>MREKGRRQAVRGPAFMFNDRGTSLTAEEERFLDAAEYGNIPVVRKMLEESKTLNVNCVDYMGQNALQLAVGNEHLEVTELLLKKENLARIGDALLLAISKGYVRIVEAILNHPGFAASKRLTLSPCEQELQDDDFYAYDEDGTRFSPDITPIILAAHCQKYEVVHMLLMKGARIERPHDYFCKCGDCMEKQRHDSFSHSRSRINAYKGLASPAYLSLSSEDPVLTALELSNELAKLANIEKEFKNDYRKLSMQCKDFVVGVLDLCRDSEEVEAILNGDLESAEPLEVHRHKASLSRVKLAIKYEVKKFVAHPNCQQQLLTIWYENLSGLREQTIAIKCLVVLVVALGLPFLAIGYWIAPCSRLGKILRSPFMKFVAHAASFIIFLGLLVFNASDRFEGITTLPNITVTDYPKQIFRVKTTQFTWTEMLIMVWVLGMMWSECKELWLEGPREYILQLWNVLDFGMLSIFIAAFTARFLAFLQATKAQQYVDSYVQESDLSEVTLPPEIQYFTYARDKWLPSDPQIISEGLYAIAVVLSFSRIAYILPANESFGPLQISLGRTVKDIFKFMVLFIMVFFAFMIGMFILYSYYLGAKVNAAFTTVEESFKTLFWSIFGLSEVTSVVLKYDHKFIENIGYVLYGIYNVTMVVVLLNMLIAMINSSYQEIEDDSDVEWKF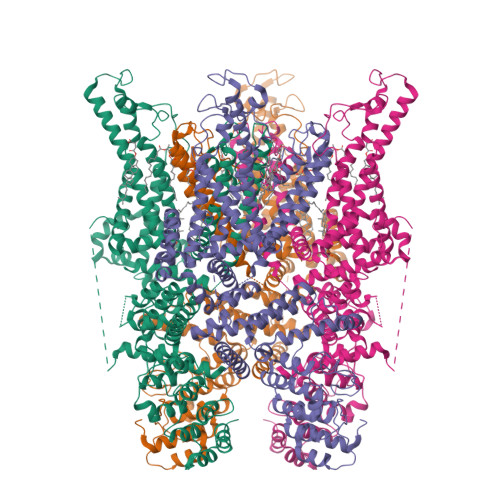ARSKLWLSYFDDGKTLPPPFSLVPSPKSFVYFIMRIVNFPKCRRRRLQKDIEMGMGNSKSRLNLFTQSNSRVFESHSFNSILNQPTRYQQIMKRLIKRYVLKAQVDKENDEVNEGELKEIKQDISSLRYELLEDKSQATEELAILIHKLSEKLNPSMLRCE[4x]L-gamma-glutamyl-S-(2-biphenyl-4-yl-2-oxoethyl)-L-cysteinylglycine | C24 H27 N3 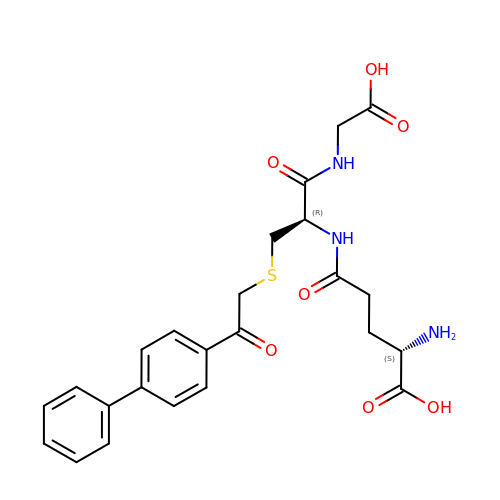O7 S | JIZFTRGOFNRYSA-OALUTQOASA-N> MIRGSSALKSLTSRRLYSTGVKYTTLSNGVTVATETNPAAKTSSVGLFFGAGSRSEHSHSNGISALTTNVLASQSAKGSLLTAKNDREFNGIIAQTTNDNITEAGKLIASIASNAVDIVEKTDLTKHKQYLSAQASAVEADPKSKVLSHLYSSAFQGYSLALPTLGTTESVENLENQDSLRHLAKHLVNNNTVIAASGNFDHDKLADAIEANLKIAEGVKPEIKPASFLGSEVRMRDDTLPKA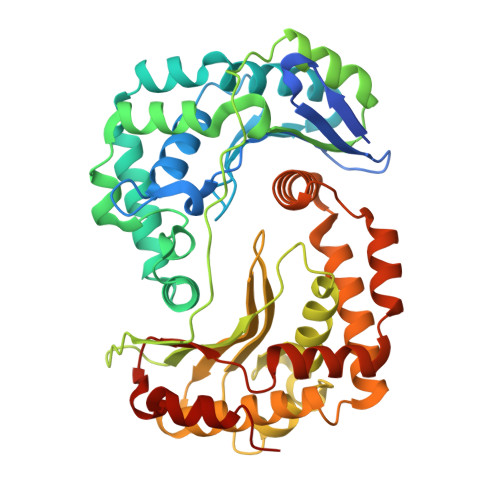YISIAVHGEGLNSPNYYLAKVAAAIYGDFYLHSTIAKFTSPKLASIVQEYNIVESYNHYSKSFSDTGIWGYYAEIADKFTVDDFTHFSLKEWNRLSISISEAEVARAKAQVKTALAKELANSFAVTSDIAEKVLLVGHRQSLREAFEKIDAIKVNDVKEWGKSKVWDRDIVISGTGLIEDLLDYNRNRNEMAMMRW3-methyl-N-[(1R)-1-(5-methyl-1,2-oxazol-3-yl)ethyl]-4-{[4-(trifluoromethyl)phenyl]methyl}-1H-pyrrole-2-carboxamide | C20 H20 F3 N3 O2 | 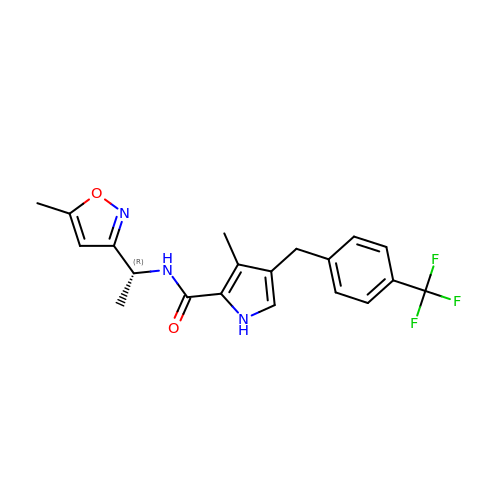GROSLFWKUCPUQW-CYBMUJFWSA-N> TDLISPVVLTNYLNSQYYGEIGIG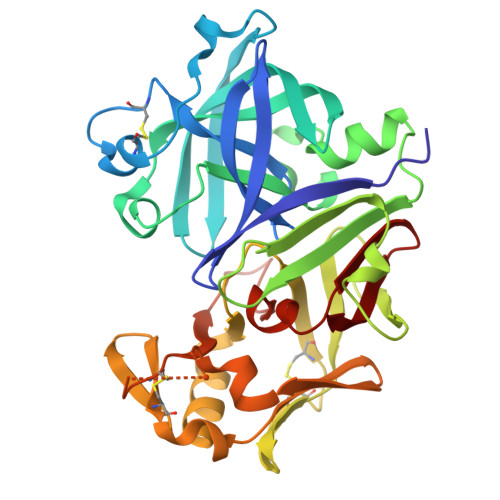TPPQTFKVIFDTGSANLWVPSTKCSRLYLACGIHSLYESSDSSSYMENGDDFTIHYGSGRVKGFLSQDSVTVGGITVTQTFGEVTQLPLIPFMLAQFDGVLGMGFPAQAVGGVTPVFDHILSQGVLKEKVFSVYYNRGPHLLGGEVVLGGSDPQHYQGDFHYVSLSKTDSWQITMKGVSVGSSTLLCEEGCEVVVDTGSSFISAPTSSLKLIMQALGAKEKRLHEYVVSCSQVPTLPDISFNLGGRAYTLSSTDYVLQYPNRRDKLCTVALHAMDIPPPTGPVWVLGATFIRKFYTEFDRHNNRIGFALAR> PNFSGNWKIIRSENFEELLKVLGVNVMLRKIWVAAASKPAVEIKQEGDTFYIKVSTTVWTTEINFKVGEEFEEQTVDGRPCKSLVKWESENKMVCEQK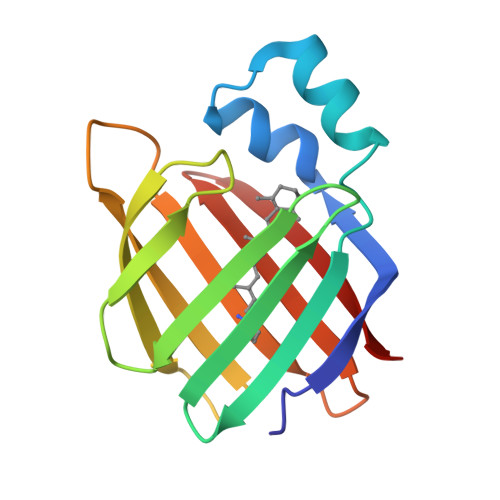LLKGEGPKTSWTKELTNDGELILTMTADDVVCTYVFVRE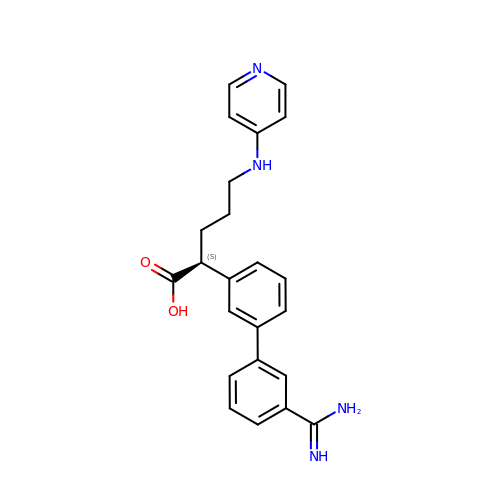(2S)-(3'-AMIDINO-3-BIPHENYL)-5-(4-PYRIDYLAMINO)PENTANOIC ACID | C23 H24 N4 O2 | FJEAIYBDDQAFGU-NRFANRHFSA-N> MAGASVKVAVRVRPFNSREMSRDSKCIIQMSGSTTTIVNPKQPKETPKSFSFDYSYWSHTSPEDINYASQKQVYRDIGEEMLQHAFEGYNVCIFAYGQTGAGKSYTMMGKQEKDQQGIIPQLCEDLFSRINDTTNDNMSYSV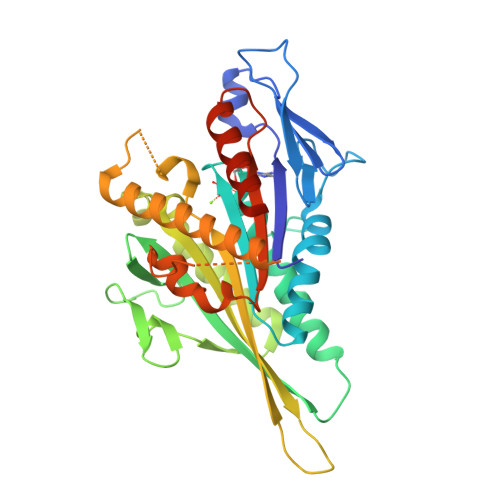EVSYMEIYCERVRDLLNPKNKGNLRVREHPLLGPYVEDLSKLAVTSYNDIQDLMDSGNKARTVAATNMNETSSRSHAVFNIIFTQKRHDAETNITTEKVSKISLVDLAGSERADSTGAKGTRLKEGANINKSLTTLGKVISALAEMDSGPNKNKKKKKTDFIPYRDSVLTWLLRENLGGNSRTAMVAALSPADINYDETLSTLRYADRAKQIRNTVSVNHHHHHH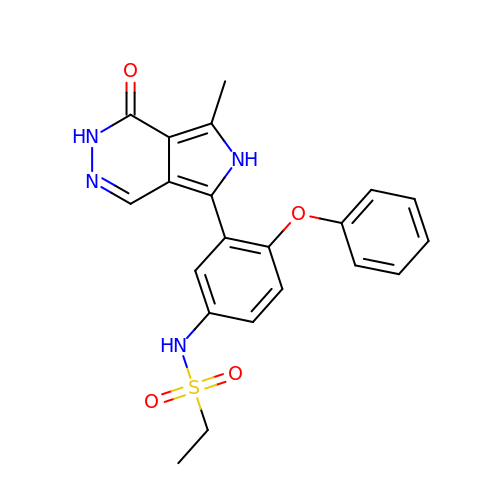N-[3-(7-methyl-1-oxo-2,6-dihydro-1H-pyrrolo[3,4-d]pyridazin-5-yl)-4-phenoxyphenyl]ethanesulfonamide | C21 H20 N4 O4 S | YYFWVXHZOKCWDD-UHFFFAOYSA-N(4R,6S,7Z,15S,17S)-17-[({7-methoxy-2-[4-(propan-2-yl)-1,3-thiazol-2-yl]quinolin-4-yl}oxy)methyl]-13-methyl-N-[(1-methylcyclopropyl)sulfonyl]-2,14-dioxo-1,3,13-triazatricyclo[13.2.0.0~4,6~]heptadec-7-ene-4-carboxamide 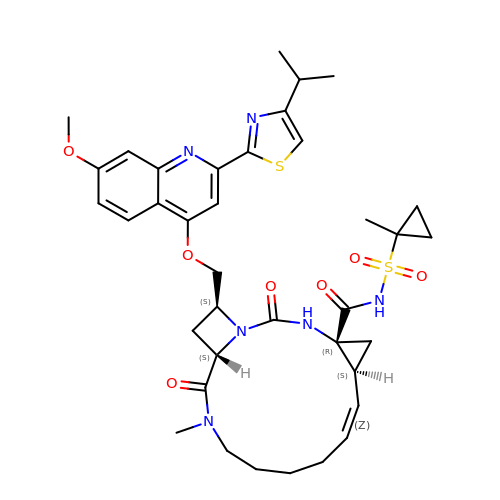| C37 H46 N6 O7 S2 | DGCPGLRWAMIHKS-GYSPVFRISA-N> GSTKERVERLC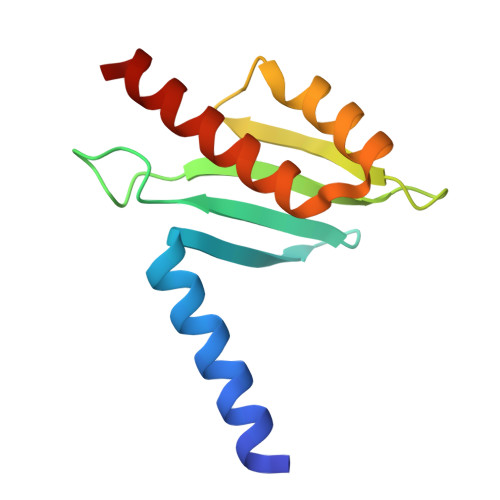KSKELFEERLGLEIRRIHNEQLQFIFRHIDHKDPDKPYMFTLSINEQGDYEVTSCTPPLDCISEFQLKVRETNNFSAFIANIRKAFTALSFKQST Chaperonins are essential protein-folding machines, classified into three structural and phylogenetic groups: Group I (bacterial GroEL), Group II (archaeal thermosome and eukaryotic CCT), and Group III (bacterial thermosome-like). All chaperonin monomers share a common three-domain structure: an apical domain involved in substrate recognition, an equatorial domain containing the ATP-binding site that drives the conformational changes that occur during the chaperonin functional cycle, and an intermediate domain linking the two by relaying signals. Using ancestral sequence reconstruction (ASR) and protein resurrection, we inferred and experimentally characterized the last common ancestors of these groups (ancestral chaperonins ACI, ACII, and ACIII). We selected several AC nodes for protein synthesis and purification, including the last common ancestors of Group I (ACI), Group II (ACII), and Group III (ACIII), along with the ancestor of the Fibrobacteres–Chlorobi–Bacteroidetes (FCB) Group (AFCB).

In the case of ACIII, oligomeric structures were visible in the absence of ATP, and they all formed double-ring structures. ACIII assembled as eight-subunit double rings without ATP-Mg²+, and AFCB formed 7-subunit double rings. The 2D classification of particles of the four ACs revealed that whereas ACI and AFCB formed heptameric rings, ACII and ACIII assembled into octameric rings, mirroring their modern counterparts. Regarding their overall structure, a typical chaperonin double-ring structure was observed for ACIII and AFCB. By contrast, ACIII and AFCB did not require ATP for either assembly or stability. Group III chaperonins, found in some bacteria, resemble Group II but lack the nucleotide-sensing loop present in Groups I and II. The remaining chaperonins E. coli GroEL, ACI and ACIII exhibited similar hydrolysis patterns. AFCB and ACIII showed similar patterns, with a small initial increase in LDH activity before stabilizing at ∼75% activity after 35 min. The evolutionary progression from an exclusively single-ring structure in ACI, to a mix of single and double rings in ACII, and finally to an exclusively double-ring assembly in ACIII, suggests a gradual, step-by-step evolution from single- to double-ring chaperonins. This pattern supports a timeline where ACI is the oldest ancestor, followed by ACII and then ACIII—with the latter likely arising through horizontal gene transfer between an ancestral archaeon and a Firmicutes bacterium rather than being a direct descendent from LUCA. For Group III ancestors, a notable increase in total stability appears to be driven by strengthened Van der Waals forces and reduced backbone clashes, indicating enhanced hydrophobic packing.

>[16x]MPLKQASSNTEADERFQALLTNVNAVRAIADAVEGTLGPKGLDVMLVDKFGEVTITNDGVTILDQMDVQHPAARMLIQVARAQEEEVGDGTTTATVLAGALVSEGVNQVEQGVPVSRVIEGLRRGVERALELLRKQALPVEGLDDPRLRAVARIAAREREDIADLVVEAARHIGEDKLQDPNFKLADTVTAREGAENQVIEGVVLNKQPLNKEMPKKLEDARVLVLDDPLEPEEIDEEALSTEAGFARYLEAQEEFRENLEKLVELGVKLVLCEKGIDDTAEELLAEAGIMAIQRVSRKDLERVAEFTGARPVKRTALNKDAEELAKLLGHAERVRYDEKLEHVCLSGGSGEPIATVLVGAATEEVVGERERVAKDAASAVQAAIRGGVVPGGGAAELAVAREVEKLAEEVKGMERYGVEAVAEALKKPLRQIVANAGFNPLEKLGDLRAAHRTGNDSLGIDCDTGEVVDMWEAGVIDPAPVKLHALKAAGEVAAAILRINTIIKMKETGPDGGEDRG N'-(3-CHLORO-4-METHOXY-PHENYL)-N-(3,4,5-TRIMETHOXYPHENYL)-1,3,5-TRIAZINE-2,4-DIAMINE 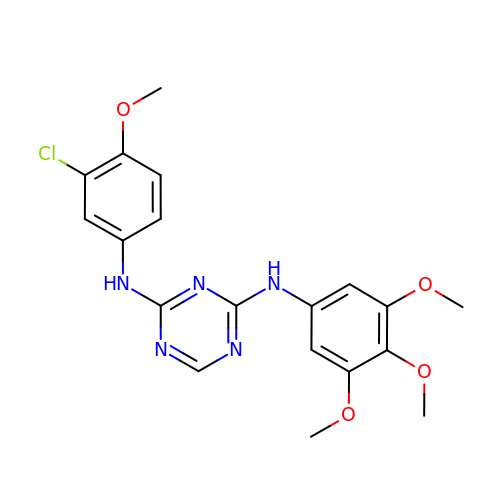| C19 H20 Cl N5 O4 | ZVWFECUPYCFYBL-UHFFFAOYSA-N>GPGSCPTHADSLNNLANIKREQGNIEEAVRLYRKALEVFPEFAAAHSNLASVLQQQGKLQEALMHYKEAIRISPTFADAYSNMGNTLKEMQDVQGALQCYTRAIQINPAFADAHSNLASIHKDSGNIPEAIASYRTALKLKPDFPDAYCNLAHCLQIVCDWTDYDERMKKLVSIVADQLEKNRLPSVHPHHSMLYPLSHGFRKAIAERHGNLCLDKINVLHKPPYEHPKDLKLSDGRLRVGYVSSDFGNHPTSHLMQSIPGMHNPDKFEVFCYALSPDDGTNFRVKVMAEANHFIDLSQIPCNGKAADRIHQDGIHILVNMNGYTKGARNELFALRPAPIQAMWLGYPGTSGALFMDYIITDQETSPAEVAEQYSEKLAYMPHTFFIGDHANMFPHLKKKAVIDFKSNGHIYDNRIVLNGIDLKAFLDSLPDVKIVKMKCPDGGDNADSSNTALNMPVIPMNTIAEAVIEMINRGQIQITINGFSISNGLATTQINNKAATGEEVPRTIIVTTRSQ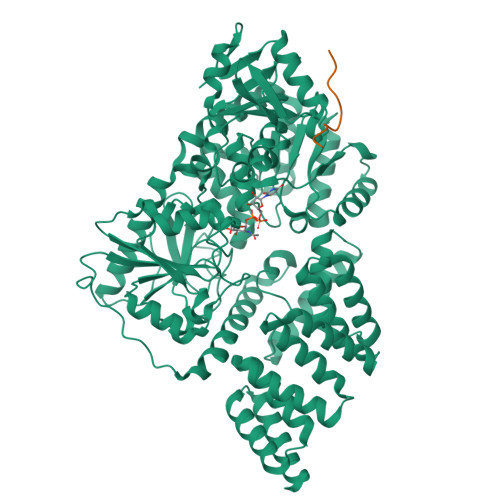YGLPEDAIVYCNFNQLYKIDPSTLQMWANILKRVPNSVLWLLRFPAVGEPNIQQYAQNMGLPQNRIIFSPVAPKEEHVRRGQLADVCLDTPLCNGHTTGMDVLWAGTPMVTMPGETLASRVAASQLTCLGCLELIAKNRQEYEDIAVKLGTDLEYLKKVRGKVWKQRISSPLFNTKQYTMELERLYLQMWEHYAAGNKPDHMIKPVE[4x];>RQFMPVYQIYLQ[4x]> HIDPESKIKDCPWYDRGFCKHGPLCR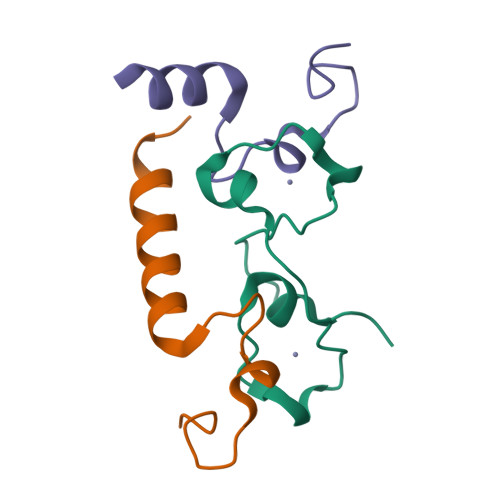HRHTRRVICVNYLVGFCPEGPSCKFMHPRFELPM;>SFEDKPWRKPGADLSDYFNYGFNEDTWKAYCEKQKRIRMGLE[2x]>ASNFTQFVLVDNGGTGDVTVAPSNFANGVAEWISSNS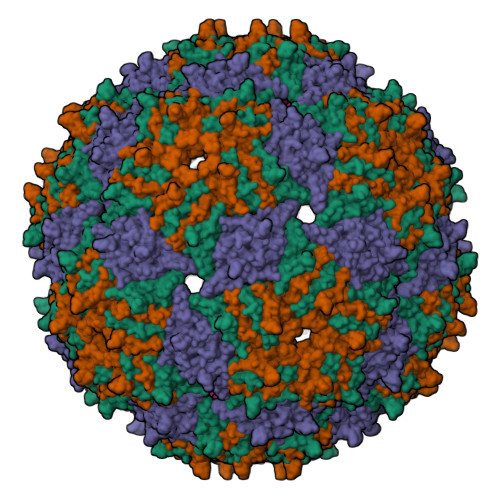RSQAYKVTCSVRQSSAQNRKYTIKVEVPKVATQTVGGVELPVAAWRSYLAMKLTIPIFATNSDCELIVKAMQGLLKDGNPIPSAIAANSGIY[3x]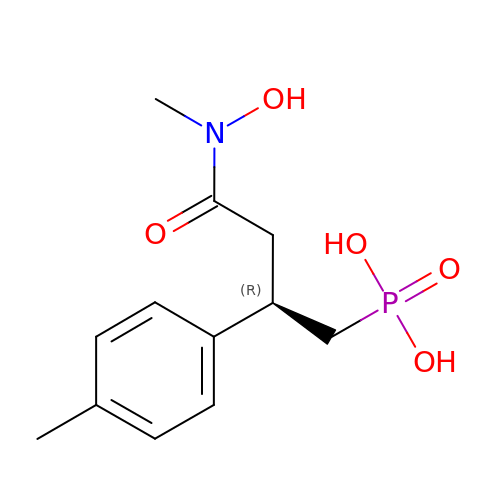[(2R)-4-[hydroxy(methyl)amino]-2-(4-methylphenyl)-4-oxobutyl]phosphonic acid | C12 H18 N O5 P | WSGLUPNSGLKEIM-NSHDSACASA-N3-(BUTYLSULPHONYL)-PROPANOIC 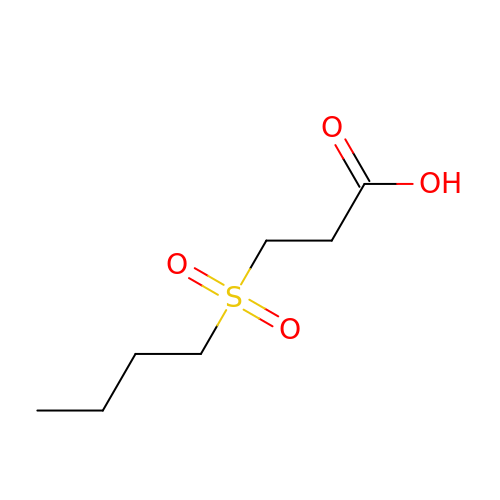ACID | C7 H14 O4 S | GSHVAQAKBLEIEY-UHFFFAOYSA-N3-[(1~{S},2~{S},5~{R})-2-carboxy-3,6-diazabicyclo[3.2.0]heptan-1-yl]propyl-$l^{3}-oxidanyl-bis(oxidanyl)boranuide | C9 H18 B N2 O5 | 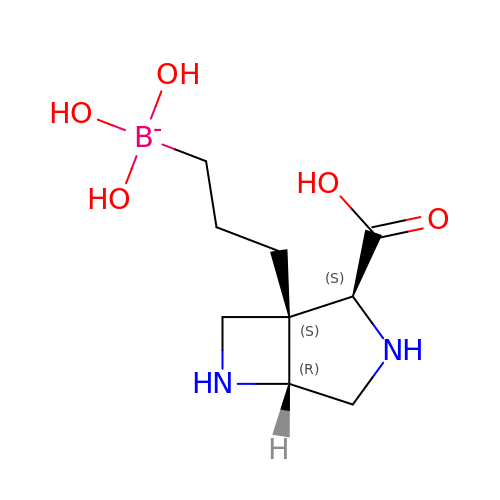BCFOBXHGEQBWQU-OOZYFLPDSA-N> LVHVASVEKGRSYEDFQKVYNAIALKLREDDEYDNYIGYGPVLVRLAWHISGTWDKHDNTGGSYGGTYRF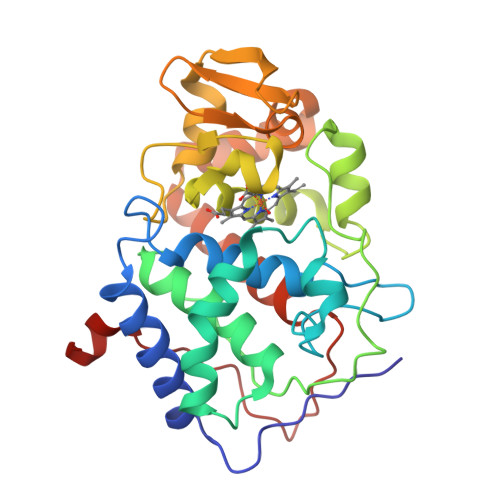KKEFNDPSNAGLQNGFKFLEPIHKEFPWISSGDLFSLGGVTAVQEMQGPKIPWRCGRVDTPEDTTPDNGRLPDADKDAGYVRTFFQRLNMNDREVVALMGAGALGKTHLKNSGYEGPWGAANNVFTNEFYLNLLNEDWKLEKNDANNEQWDSKSGYMMLPTDYSLIQDPKYLSIVKEYANDQDKFFKDFSKAFEKLLENGITFPKDAPSPFIFKTLEEQGL TETRAHYDROURIDINE | C9 H16 N2 O6 | 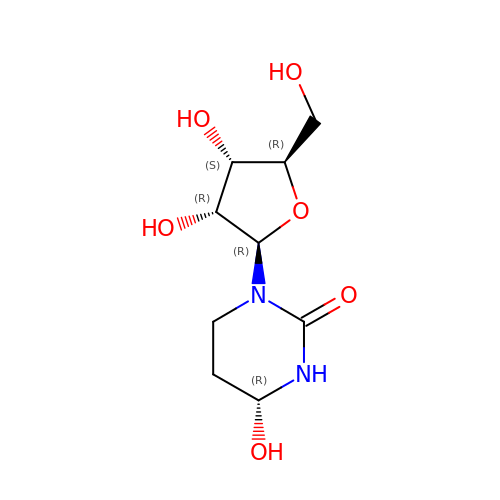UCKYOOZPSJFJIZ-FMDGEEDCSA-N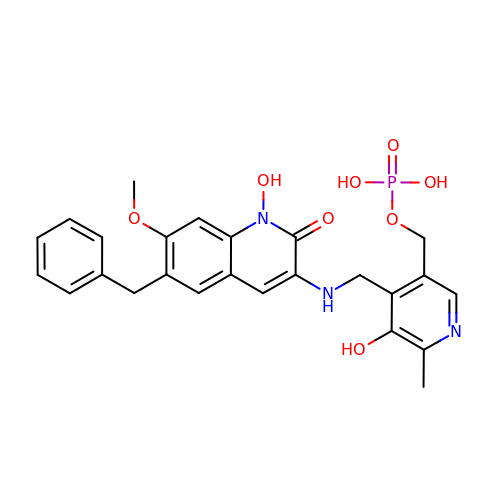(4-{[(6-benzyl-1-hydroxy-7-methoxy-2-oxo-1,2-dihydroquinolin-3-yl)amino]methyl}-5-hydroxy-6-methylpyridin-3-yl)methyl dihydrogen phosphate | C25 H26 N3 O8 P | XUOFFKSMLSNCMV-UHFFFAOYSA-N>[8x]MSLKITEVKAHALSTPIPERMRVESGAGLKLNRQMI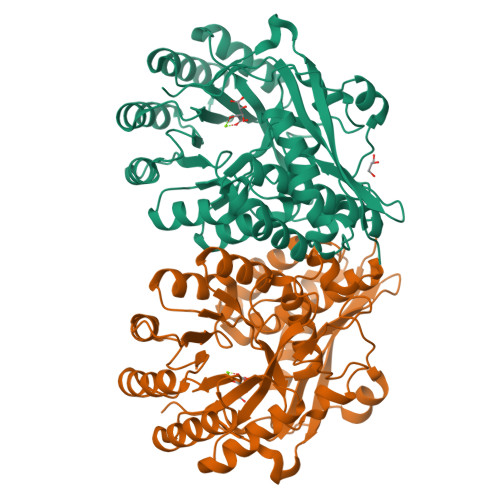LVEVRTDEGVTGVGSPSGPYDLAVLKRAIEDVIGPQLIGEDPANINYLWHKVFHGEVSRNLGHRSVGIAAMSGVDIALWDLKGRAMNQPIYQLLGGKFHTRGVRAYASSIYWDLTPDQAADELAGWVEQGFTAAKLKVGRAPRKDAANLRAMRQRVGADVEILVDANQSLGRHDALAMLRILDEAGCYWFEEPLSIDDIEGHRILRAQGTPVRIATGENLYTRNAFNDYIRNDAIDVLQADASRAGGITEALAISASAASAHLAWNPHTFNDIITVAANLHLVAASPHPAMFEWDITHNDLMTRLASYDLKLENGLVQPPQGPGLGFEIDWDFVAAHAWKGEPAIGAGHGMKK4-hydroxy-8-sulfoquinoline-3-carboxylic acid 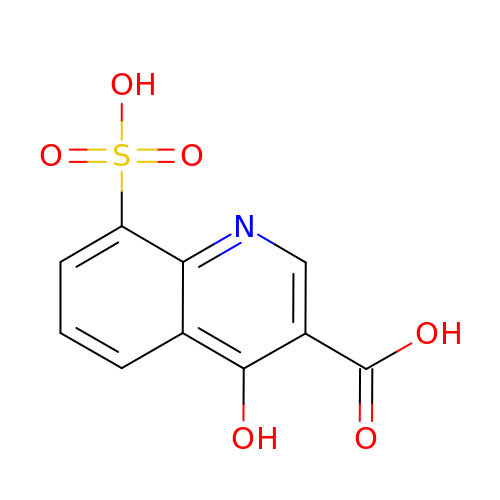| C10 H7 N O6 S | FKTVHRZETGCILU-UHFFFAOYSA-N> MLEVCIIGFGFSAIPLVRELARTQTEFQIISAESGSVWDRLSESGRLDFSLVSSFQTSFYSFDLVRDYEKDYYPTAKQFYEMHERWRSVYEEKIIRDFVTKIENFKDYSLISTRSGKTYEAKHVVLATGFDRLMNTFLSNFDNHVSNKTFVFDTMGDSANLLIAKLIPNNNKIILRTNGFTALDQEVQVLGKPFTLDQLESPNFRYVSSELYDRLMMSPVYPRTVNPAVSYNQFPLIRRDFSWVDSKSSPPNGLIAIKYWPIDQYYYHFNDDLENYISKGYLLNDIAMWLHTGKVILVPSDTPINFDKKTITYAGIERSFHQYVKGDAEQPRLPTILINGETPFEYLYRDTFMGVIPQRLNNIYFLGYTRPFTGGLANITEMQSLFIHKLITQPQFHQKIHQNLSKRITAYNQHYYGAAKPRKHDHTVPFGFYTEDIARLIGIHYQPNECRSVRDLLFYYAFPNNAFKYRLKGEYAVDGVDELIQKVNDKHDHYAQVFVQALSIRNMNSDEAAEWDHSARRFAFNDMRHKEGYRAFLDTYLKAYRQVENISVDDTVVDEEWNFMVKEACQVRDKVAPNIEEKTHYSKDEDVNKGIRLILSILDSDISSLPDSNGSRGSGNLKEGDRLCKFEAQSIEFIRRLLQPKNYELLFIRESTVSPGSHRHGETA

The first documented single-component Trp-FDH is AetF from cyanobacterium *Aetokthonos hydrillicola*, which catalyzes consecutively bromination on C5 and then C7 of Trp to generate 5,7-di-Br-Trp. More recently, a class of “single-component” FDHs has been identified. These enzymes fuse pyridine nucleotide-dependent flavin reductase and FDH on the same polypeptide chain, an advantageous feature in the application aspect relative to canonical FDHs owing to the omission of including a flavin reductase. The action of FDHs requires the reduced flavin and molecular oxygen to generate hydroperoxyl flavin intermediate, which oxidizes a halide ion to form a halogenating reagent hypohalous acid (HOX). The flipping allows the carbon-to-be-halogenated to be oriented toward the catalytic residue K258 and within the hydrogen bond distance to the putative general base E200, such that the halogenation site on two substrates is switched from C5 to C7.

When conducting Ala substitution to investigate the role of the substrate-binding residues in our previous study, we found that substituting S523, a residue that binds the carboxyl group of the substrate, to Ala leads to 2.5-fold increase in 5-Br-Trp production and very low di-brominated product. Before conducting engineering, the crystal structure of AetF-S523A in complex with Trp was resolved (**[Table tbl1]**). The electron density maps corresponding to Trp were clearly observed in the substrate-binding pocket (**[Fig fig1]**). The binding pose and the interaction network of Trp to the enzyme are identical to those of the wild type enzyme (**[Fig fig1]**). This indicates that removing S523-mediated polar interaction poses minimal influence to the binding of Trp. Noteworthily, we failed to obtain the complex structure of AetF-S523A and 5-Br-Trp despite of great efforts, which should be attributed to the low affinity of the variant enzyme to the compound. This also indicates that the S523-mediated interaction is crucial to the binding of 5-Br-Trp, such that the Ala substitute is incapable of accepting the substrate that shows a flipped pose relative to Trp and displays low dibrominated Trp production activity as previously proposed. It should be noted that AetF-S523A still produces trace amounts of 5,7-di-Br-Trp (**[Fig fig1]**). AetF-S523A, a variant that was identified in our previous study, exhibits around 3.9 % activity to produce di-brominate Trp compared with the wild type enzyme.> MRPYYIAIVGSGPSAFFAAASLLKAADTTEDLDMAVDMLEMLPTPWGLVRSGVAPDQPKIKSISKQFEKTAEDPRFRFFGNVVVGEHVQPGELSERYDAVIYAVGAQSDRMLNIPGEDLPGSIAAVDFV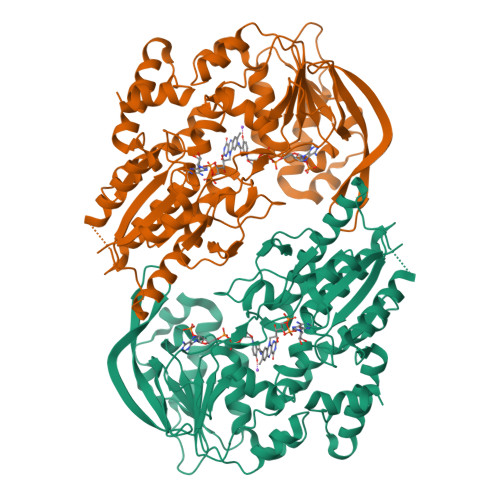GWYNAHPHFEQVSPDLSGARAVVIGNGNVALDVARILLTDPDVLARTDIADHALESLRPRGIQEVVIVGRRGPLQAAFTTLELRELADLDGVDVVIDPAELDGITDEDAAAVGKVCKQNIKVLRGYADREPRPGHRRMVFRFLTSPIEIKGKRKVERIVLGRNELVSDGSGRVAAKDTGEREELPAQLVVRSVGYRGVPTPGLPFDDQSGTIPNVGGRINGSPNEYVVGWIKRGPTGVIGTNKKDAQDTVDTLIKNLGNAKEGAECKSFPEDHADQVADWLAARQPKLVTSAHWQVIDAFERAAGEPHGRPRVKLASLAELLRIGLG~{N}-(furan-2-ylmethyl)-4-methyl-piperidine-1-carboxamide 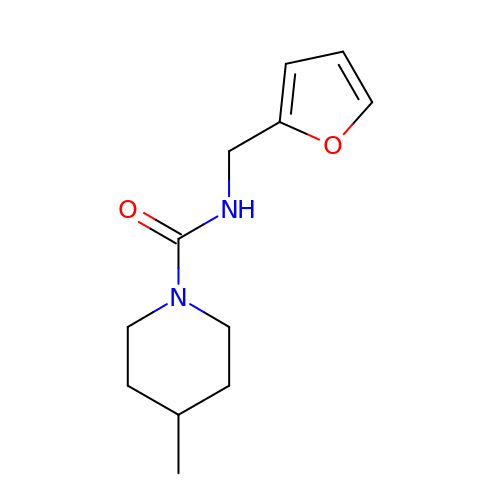| C12 H18 N2 O2 | WVQSALJZZLSNAY-UHFFFAOYSA-N> SMAALAPLPPLPAQFKSIQHHLRTAQEHDKRDPVVAYY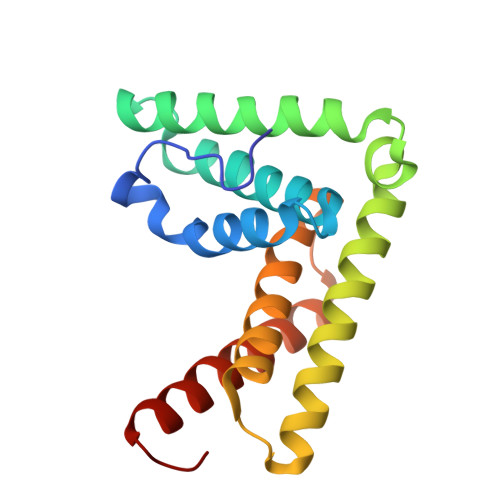CRLYAMQTGMKIDSKTPECRKFLSKLMDQLEALKKQLGDNEAITQEIVGCAHLENYALKMFLYADNEDRAGRFHKNMIKSFYTASLLIDVITVFGELTDENVKHRKYARWKATYIHNCLKNGETP> MDLEKNYPTPRTSRTGHGGVNQLGGVFVNGRPLPDVVRQRIVELAHQGVRPCDISR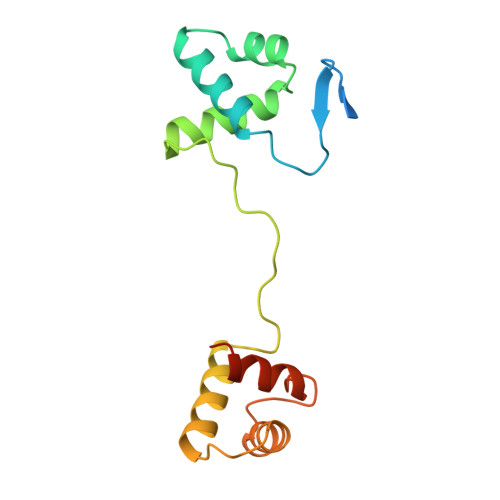QLRVSHGCVSKILGRYYETGSIKPGVIGGSKPKVATPKVVEKIAEYKRQNPTMFAWEIRDRLLAERVCDNDTVPSVSSINRIIRTKVQQPPNQ> DSKKIVGVFYKANEYATKNPNFLGCVENALGIRDWLESQGHQYIVTDDKEGPDCELEKHIPDLHVLISTPFHPAYVTAERIKKAKNLKLLLTAGIGSDHIDLQAAAAAGLTVAEVTGSNVVSVAEDELMRILILMRNFVPGYNQVVKGEWNVAGIAYRAYDLEGKTIGTVGAGRIGKLLLQR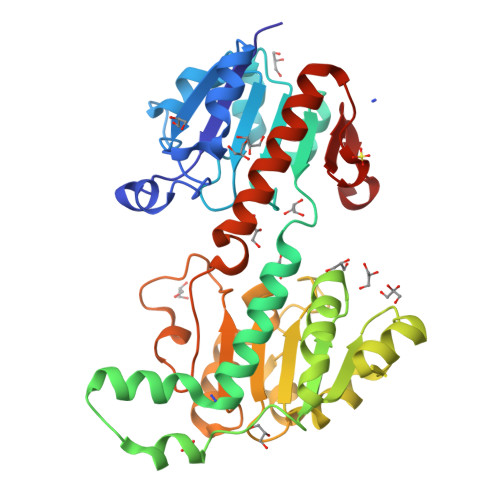LKPFGCNLLYHDRLQMAPELEKETGAKFVEDLNEMLPKCDVIVINMPLTEKTRGMFNKELIGKLKKGVLIVNNARGAIMERQAVVDAVESGHIGGYSGDVWDPQPAPKDHPWRYMPNQAMTPHTSGTTIDAQLRYAAGTKDMLERYFKGEDFPTENYIVKDGELAPQYR> MSVSSIISHAQFDRMLLHRNDGACQAKGFYTYDAFVAAANAFPGFGATGSTDARKRDVAAFLAQTSHQTTGGAATAPDGAFAWGYCFKQERGAAADYCTPSAQWPCAPGKRYYGRGPIQLSHNYNYGPAGRAIGVDLLRNPDLVATDPTVSFKTALWFWMTAQAPKPS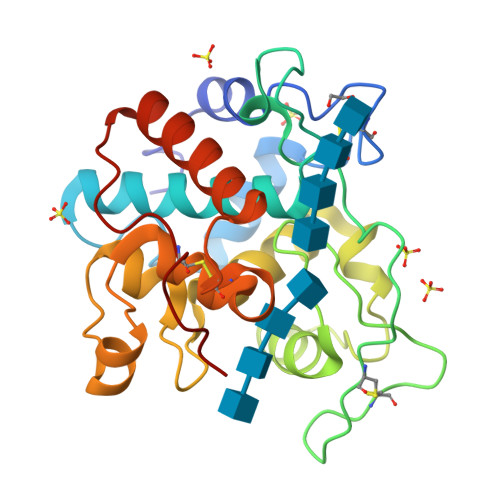SHAVITGKWSPSGADRAAGRAPGFGVITNIINGGLECGHGQDSRVADRIGFYKRYCDILGVGYGDNLDCYNQRPFA The 12 related human ESCRT-III proteins form filaments that constrict membranes and mediate fission, including during cytokinetic abscission. Human ESCRT-III proteins have conserved helical core domains that mediate filament formation, and variable C-terminal tails that contain short peptide elements called MIT-Interacting Motifs (MIMs). MIMs bind cofactors that contain MIT (Microtubule-Interacting and Trafficking) domains (Hurley and Yang, 2008). MIT domains are simple three helix bundles, but they can bind MIM elements in at least seven distinct ways (Skalicky et al., 2012; Obita et al., 2007; Scott et al., 2005; Stuchell-Brereton et al., 2007; Kieffer et al., 2008, Yang et al., 2008; Solomons et al., 2011; Fujioka et al., 2014), which we have termed Type 1–7 binding modes.

The MIT domain of the microtubule severing AAA+ ATPase SPASTIN binds CHMP1B, which reportedly localizes the enzyme to the midbody where it clears spindle microtubules to allow abscission. The SPASTIN MIT domain is unusual in binding specifically to three different ESCRT-III proteins: CHMP1B, CHMP3, and IST1. We determined a high resolution (1.15 Å) crystal structure of the SPASTIN MIT-IST1 complex using a SPASTIN MIT112-196 construct. The structure revealed that the IST1 MIM344-366 adopts an amphipathic helix that buries its hydrophobic side chains in the SPASTIN MIT H1/H3 groove (Type 3 binding). Four hydrophobic IST1 residues, F352, L355, F359, and L362 are shown binding in the H1/H3 groove of the SPASTIN MIT domain. The interface buries 1400 Å2 of surface area over 32 residues from both faces and is further stabilized with four hydrogen bonds and seven salt bridges. The IST1 and CHMP1B MIM elements exhibit similar binding modes, but with two significant differences: (1) The longer CHMP1B helix extends three additional turns beyond the IST1 N-terminus, and (2) the MIT H1/H3 groove expands to accommodate the longer CHMP1B helix, with a maximal displacement of 2.5 Å at the N-terminus of helix 3. IST1 binding is slightly tighter than CHMP1B binding, likely owing to enhanced hydrophobic interactions with the SPASTIN H1/H3 groove. IST1 buries two aromatic and two aliphatic side chains, whereas the CHMP1B binding element lacks aromatic residues and buries only three aliphatics.

> EAERVRVFHKQAFEYISIALRIDEDEKAGQKEQAVEWYKKGIEELEKGIAVIVTGQGEQCERARRLQAKMMTNLVMAKDRLQLL;> TSASEDIDFDDLSRRFEELKKKT> MDEAVGDLKQALPCVAESPTVHVEVHQRGSSTAKKEDINLSVRKLLNRHNIVFGDYTWTEFDEPFLTRNVQSVSIIDTELKVKDSQPIDLSACTVALHIFQLNEDGPSSENLEEETENIIAANHWVLPAAEFHGLWDSLVYDVEVKSHLLDYVMTTLLFSDKNVNSNL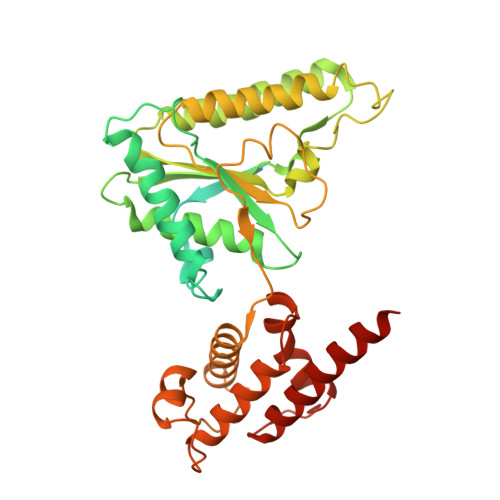ITWNRVVLLHGPPGTGKTSLCKALAQKLTIRLSSRYRYGQLIEINSHSLFSKWFSESGKLVTKMFQKIQDLIDDKDALVFVLIDQVESLTAARNACRAGTEPSDAIRVVNAVLTQIDQIKRHSNVVILTTSNITEKIDVAFVDRADIKQYIGPPSAAAIFKIYLSCLEELMKCQIIYPRQQLLTLRELEMIGFIENNVSKLSLLLNDISRKSEGLSGRVLRKLPFLAHALYVQAPTVTIEGFLQALSLAVDKQFEERKKLAAYI>GSHMSQSLFSLAFGVGTQNRQEAWLEVFYALPLLKPSSEIVAAVAPILGYAAGNQALTFTSQQAYQLADALKGIDAAQSALLSRLAESQKPLVATLLAEDAAPSSTAEAYLKLHLLSHRLVKPHAVNLSGIFPLLPNVAWTNIGAVDLAELAELQLEARLKGKLLEVFSVDKFPKMTDYVVPAGVRIADTARVRLGAYIGEGTTVMHEGFVNFNAGTEGPGMIEGRVSAGVFVGKGSDLGGGCSTMGTLSGGGNIVISVGEGCLIGANAGIGIPLGDRNIVEAGLYITAGTKVALLDEQNALVKVVKARDLAGQPDLLFRRNSQNGAVECKTNKTAIELNEALHAHN[6x]

Pseudomonas aeruginosa is an opportunistic pathogen that causes persistent infections in humans. Randomized transposon mutagenesis screens had indicated several genes from the diaminopimelate (DAP) biosynthetic pathway to lysine in P. aeruginosa as essential, suggesting the corresponding gene products as potential targets for new antibacterial drugs. Dihydrodipicolinate synthase (DapA) catalyzes the first committed step of the DAP pathway, the condensation of L-aspartate-semialdehyde and pyruvate to 4-hydroxy-2,3,4,5-tetrahydro-L,L-dipicolinic acid, which is non-enzymatically dehydrated to yield L-2,3-diydrodipicolinate. Tetrahydrodipicolinate N-succinyltransferase (DapD) catalyses the transfer of the succinyl moiety of succinyl-CoA to the α-amino group of tetrahydrodipicolinate, the first committed step in the succinylase branch of the DAP biosynthesis pathway present in most Gram-negative bacteria and mycobacteria.

The reaction is stereospecific with respect to the amino donor substrate, i.e. only L-2 aminopimelate was accepted as substrate with a KM of 7.0 mM and a Vmax of 105 µmol/min. Eventually, these complexes could be prepared by soaking of monoclinic crystals of PaDapD in crystallisation liquor, where succinate had been replaced with either L- or D-2-aminopimelate. The crystallographic binding studies with the amino donor substrate L-2-AP allowed straightforward fitting of the substrate in the active sites of all subunits with the exception of chain B, where the electron density is too weak for unambiguous modelling of bound L-2-AP, indicating lower occupancy of the ligand. In three of the subunits (chains A, D and E) the binding mode of the substrate is very similar to those seen with its stereoisomer, D-2-aminopimelate. The ε-carboxyl group of L-2AP forms salt bridges with the guanidinium groups of residues Arg18 and Arg19 and the α-carboxylate of L-2AP forms hydrogen bonds to the side chain of Asn209 and the main chain amino group of Ala226. In addition, the α-amino group of L-2AP is also within hydrogen binding distance to the side chain of Glu221. A comparison of the PaDapD-L-2AP binary complex with the structure of the ternary complex of the E. coli enzyme with coenzyme A and L-2AP reveals a very similar binding mode and conserved enzyme-ligand interactions in both enzymes. The binding of the substrate to the remaining two active sites (C and F) is somewhat different from the one observed in chains A, D, and E and can best be described as intermediate binding steps. While the tail carboxyl group and parts of the alkyl chain of L-2-AP are inserted into the active site, with the interactions of the carboxyl tail to the two arginine residues Arg181 and Arg193 formed, the remaining part of the carbon chain and the head group is still in contact with the bulk solution and does not yet interact with protein residues.> IVGGYTCAANSIPYQVSLNSGSHFCGGSLINSQWVVSAAHCYKSRIQVRLGEHNIDVLEGNEQFINAAKII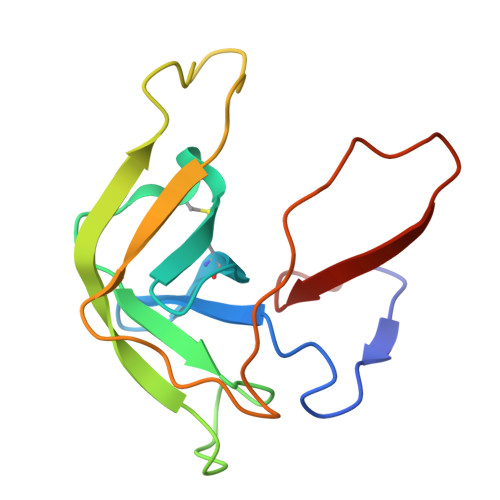THPNFNGNTLDNDIMLIKLSSPATLNSRVATVSLPRSCAAAGTECLISGWGNTK> LVKEEIQAKEYLENLNKELAKRTNVETEAAWAYGSNITDENEKKKNEISAELAKFMKEVASDTTKFQWRSYQSEDLKRQFKALTKLGYAALPEDDYAELLDTLSAMESNFAKVKVCDYKDSTKCDLALDPEIEEVISKSRDHEELAYYWREFYDKAGTAVRSQFERYVELNTKAAKLNNF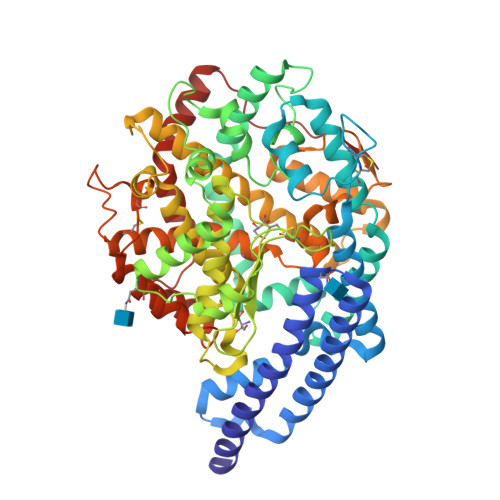TSGAEAWLDEYEDDTFEQQLEDIFADIRPLYQQIHGYVRFRLRKHYGDAVVSETGPIPMHLLGNMWAQQWSEIADIVSPFPEKPLVDVSAEMEKQGYTPLKMFQMGDDFFTSMNLTKLPQDFWDKSIIEKPTDGRDLVCHASAWDFYLTDDVRIKQCTRVTQDQLFTVHHELGHIQYFLQYQHQPFVYRTGANPGFHEAVGDVLSLSVSTPKHLEKIGLLKDYVRDDEARINQLFLTALDKIVFLPFAFTMDKYRWSLFRGEVDKANWNCAFWKLRDEYSGIEPPVVRSEKDFDAPAKYHISADVEYLRYLVSFIIQFQFYKSACIKAGQYDPDNVELPLDNCDIYGSAAAGAAFHNMLSMGASKPWPDALEAFNGERIMSGKAIAEYFEPLRVWLEAENIKNNVHIGWTTSNKCVSS> MAQNPFKALNINIDKIESALTQNGVTNYSSNVKNERETHISGTYKGIDFLIKLMPSGGNTTIGRASGQNNTYFDEIALIIKENCLYSDTKNFEYTIPKFSDDDRANLFEFLSEE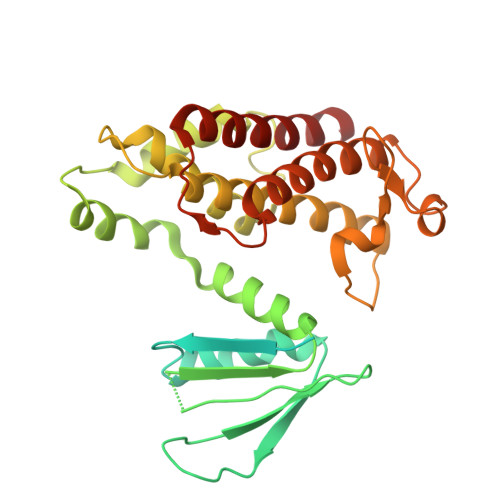GITITEDNNNDPNCKHQYIMTTSNGDRVRAKIYKRGSIQFQGKYLQIASLINDFMCSILNMKEIVEQKNKEFNVDIKKETIESELHSKLPKSIDKIHEDIKKQLSCSLIMKKIDVEMEDYSTYCFSALRAIEGFIYQILNDVCNPSSSKNLGEYFTENKPKYIIREIHQETINGEIAEVLCECYTYWHENRHGLFHMKPGIADTKTINKLESIAIIDTVCQLIDGGVARLKL>[4x]GPGSMKLYDFEVGLDQPFFLIAGTCVVESEQMTIDTAGRLKEICAKLNVPFIYKSSYDKANRSSGKSFRGLGMDEGLRILGEVKRQLGLPVLTDVHSIDEIEQVASVVDVLQTPAFLCRQTDFIHACARSGKPVNIKKGQFLAPHDMKNVIDKAREAAREAGLSEDRFMACERGVSFGYNNLVSDMRSLAIMRETSAPVVFDATHSVQLPGGQGTSSGGQREFVPVLARAAVATGVAGLFMETHPNPAEAKSDGPNAVPLNRMGALLETLVTLDQAVKRHPFLENDFN

Here we report a functional and structural genomics effort that applied saturation-level transposon mutagenesis and next generation sequencing (Tn-seq) to identify essential genes in B. thailandensis, followed by high-throughput structure determination. We used an “ortholog rescue” approach to maximize structural coverage of these gene families, which are likely to be essential not only in B. thailandensis, but also in related, but more virulent, Burkholderia species, such as B. pseudomallei. Using only seven Burkholderia species to select orthologs of essential genes, we solved structures for 49/406 essential gene families, and for 56 total Burkholderia protein targets (including seven ortholog replicates). Of these 56 targets, 25 satisfied criteria for being a potential antimicrobial drug target.

By using an ortholog rescue strategy for insoluble or difficult to crystallize targets, we increased our structural coverage of B. thailandensis essential genes from 31/406 (7.6%) to 49/406 (12.1%). For the seven pairs of ortholog structures (with no bound ligand) solved in this study, the average overall Cα RMSD was 1.5±0.5 Å, indicating a high degree of structural similarity. This structural similarity suggests that the ortholog approach is an efficient method to obtain useable structures from otherwise intractable targets, thereby lowering the barrier to structure-based drug design targeting infectious organisms.>TADELVFFVNGKKVVEKNADPETTLLAYLRRKLGLRGTKLGCGEGGCGACTVMLSKYDRLQDKIIHFSANACLAPICTLHHVAVTTVEGIGSTKTRLHPVQERIAKSHGSQCGFCTPGIVMSMYTLLRNQPEPTVEEIEDAFQGNLCRCTGYRPILQGFRTFAKNGGCCGGNGNNPNCCMNQKKDHTVTLSPSLFNPEEFMPLDPTQEPIFPPELLRLKDVPPKQLRFEGERVTWIQASTLKELLDLKAQHPEAKLVVGNTEIGIEMKFKNQLFPMIICPAWIPELNAVEHGPEGISFGAACALSSVEKTLLEAVAKLPTQKTEVFRGVLEQLRWFAGKQVKSVASLGGNIITASPISDLNPVFMASGTKLTIVSRGTRRTVPMDHTFFPSYRKTLLGPEEILLSIEIPYSREDEFFSAFKQASRREDDIAKVTCGMRVLFQPGSMQVKELALCYGGMADRTISALKTTQKQLSKFWNEKLLQDVCAGLAEELSLSPDAPGGMIEFRRTLTLSFFFKFYLTVLKKLGKDSKDKCGKLDPTYTSATLLFQKHPPANIQLFQEVPNGQSKEDTVGRPLPHLAAAMQASGEAVYCDDIPRYENELFLRLVTSTRAHAKIKSIDVSEAQKVPGFVCFLSADDIPGSNETGLFNDETVFAKDTVTCVGHIIGAVVADTPEHAERAAHVVKVTYEDLPAIITIEDAIKNNSFYGSELKIEKGDLKKGFSEADNVVSGELYIGGQDHFYLETHCTIAIPKGEEGEMELFVSTQNAMKTQSFVAKMLGVPVNRILVRVKRMGGGFGGKETRSTLVSVAVALAAYKTGHPVRCMLDRNEDMLITGGRHPFLARYKVGFMKTGTIVALEVDHYSNAGNSRDLSHSIMERALFHMDNCYKIPNIRGTGRLCKTNLSSNTAFRGFGGPQALFIAENWMSEVAVTCGLPAEEVRWKNMYKEGDLTHFNQRLEGFSVPRCWDECLKSSQYYARKSEVDKFNKENCWKKRGLCIIPTKFGISFTVPFLNQAGALIHVYTDGSVLVSHGGTEMGQGLHTKMVQVASKALKIPISKIYI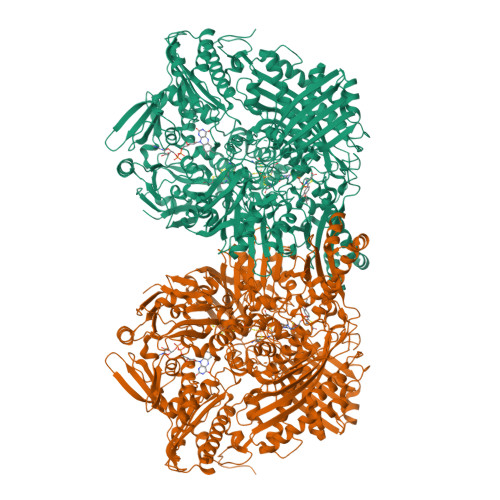SETSTNTVPNSSPTAASVSTDIYGQAVYEACQTILKRLEPFKKKNPDGSWEDWVMAAYQDRVSLSTTGFYRTPNLGYSFETNSGNAFHYFTYGVACSEVEIDCLTGDHKNLRTDIVMDVGSSLNPAIDIGQVEGAFVQGLGLFTLEELHYSPEGSLHTRGPSTYKIPAFGSIPTEFRVSLLRDCPNKKAIYASKAVGEPPLFLGASVFFAIKDAIRAARAQHTNNNTKELFRLDSPATPEKIRNACVDKFTTLCVTGAPGNCKPWSLRV[2x]The ubiquitin system, composed of ubiquitin-activating enzyme (E1), ubiquitin-conjugating enzyme (E2), and ubiquitin ligase (E3), regulates numerous cellular functions through the generation of various ubiquitin chains in a system referred to as the ubiquitin code. HOIP, as well as HOIL-1L, belongs to the RBR-type E3 family, and the family E3s reportedly generate polyubiquitin chains through a RING-HECT-hybrid reaction. Among them, HOIP contains the E3 active site. The linear ubiquitin chain functions as a scaffold to recruit other IκB kinase (IKK) molecules, and the recruited IKK molecules are then activated by a trans-phosphorylation mechanism, leading to the activation of the NF-κB signaling pathway.

We identified a thiol-reactive, α,β-unsaturated carbonyl-containing chemical compound, named HOIPIN-1 from HOIP inhibitor-1, as a LUBAC inhibitor. In the presence of HOIPIN-1, the molecular mass of the truncated HOIP increased by 263. This suggested that HOIPIN-1 stoichiometrically binds to HOIP. Collectively, these results indicated that HOIPIN-1 selectively suppresses the RING-HECT-hybrid reaction of LUBAC, as represented by the thioester-linked donor ubiquitin transfer from E2 to the active Cys885 of HOIP. HOIPINs are covalently attached to the catalytic Cys885 of HOIP via Michael addition. The benzoate moiety of HOIPINs is the key element for binding to HOIP. The carboxyl group of the benzoate hydrogen bonds with Arg935, and the aromatic ring of the benzoate hydrophobically interacts with Phe905, Leu922, and the aliphatic portion of His887. The aromatic ring of the methoxyphenyl moiety of HOIPIN-1 and the 2,6-difluorophenyl moiety of HOIPIN-8 stack on the carboxyl group of the benzoate moiety and the guanidino group of Arg935, respectively. The HOIPIN-1- and HOIPIN-8-bound structures of HOIP explain the differences in the inhibition activities of the eight HOIP inhibitors with petit-LUBAC. Indeed, a structural analysis clearly indicated that not only the RING2 domain but also the unique residues in the LDD domain, such as Arg935 and Asp936, contribute to the binding-specificity of HOIPINs to LUBAC.

> GPGHMPEYQAQGLAMYLQENGIDCPKCKFSYALARGGCMHFHCTQCRHQFCSGCYNAFYAKNKCPEPNCRVKKSLHGHHPRDCLFYLRDWTALRLQKLLQDNNVMFNTEPPAGARAVPGGGCRVIEQKEVPNGLRDEACGKETPAGYAGLCQAHYKEYLVSLINAHSLDPATLYEVEELETATERYLHVRPQPLAGEDPPAYQARLLQKLTEEVPLGQSIPRRRK> MSGAAAASAAGYDRHITIFSPEGRLYQVEYAFKATNQTNINSLAVRGKDCTVVISQKKVPDKLLDPTTVSYIFCISRTIGMVVNGPIPDARNAALRAKAEAAEFRYKYGYDMPCDVLAKRMANLSQIYTQRAYMRPLGVILTFVSVDEELGPSIYKTDPAGYYVGYKATATGPKQQEITTNLENHFKKSKIDHINEESWEKVVEFAITHMIDALGTEFSKNDLEVGVATKDKFFTLSAENIEERLVAIAEQD;> MTDRYSFSLTTFSPSGKLGQIDYALTAVKQGVTSLGIKATNGVVIATEKKSSSPLAMSETLSKVSLLTPDIGAVYSGMGPDYRVLVDKSRKVAHTSYKRIYGEYPPTKLLVSEVAKIMQEATQSGGVRPFGVSLLIAGHDEFNGFSLYQVDPSGSYFPWKATAIGKGSVAAKTFLEKRWNDELELEDAIHIALLTLKESVEGEFNGDTIE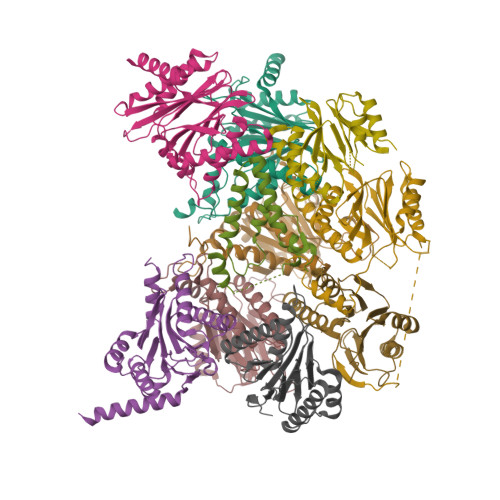LAIIGDENPDLLGYTGIPTDKGPRFRKLTSQEINDRLEAL;> MGSRRYDSRTTIFSPEGRLYQVEYALESISHAGTAIGIMASDGIVLAAERKVTSTLLEQDTSTEKLYKLNDKIAVAVAGLTADAEILINTARIHAQNYLKTYNEDIPVEILVRRLSDIKQGYTQHGGLRPFGVSFIYAGYDDRYGYQLYTSNPSGNYTGWKAISVGANTSAAQTLLQMDYKDDMKVDDAIELALKTLSKTTDSSALTYDRLEFATIRKGANDGEVYQKIFKPQEIKDILVKTGITKKDEDEEADEDMK;> MSGYDRALSIFSPDGHIFQVEYALEAVKRGTCAVGVKGKNCVVLGCERRSTLKLQDTRITPSKVSKIDSHVVLSFSGLNADSRILIEKARVEAQSHRLTLEDPVTVEYLTRYVAGVQQRYTQSGGVRPFGVSTLIAGFDPRDDEPKLYQTEPSGIYSSWSAQTIGRNSKTVREFLEKNYDRKEPPATVEECVKLTVRSLLEVVQTGAKNIEITVVKPDSDIVALSSEEINQYVTQIEQEKQEQQEQDKKKKSNH;> MTSIGTGYDLSNSVFSPDGRNFQVEYAVKAVENGTTSIGIKCNDGVVFAVEKLITSKLLVPQKNVKIQVVDRHIGCVYSGLIPDGRHLVNRGREEAASFKKLYKTPIPIPAFADRLGQYVQAHTLYNSVRPFGVSTIFGGVDKNGAHLYMLEPSGSYWGYKGAATGKGRQSAKAELEKLVDHHPEGLSAREAVKQAAKIIYLAHEDNKEKDFELEISWCSLSETNGLHKFVKGDLLQEAIDFAQKEINGDDDEDEDDSDNVMSSDDENAPVATNANATTDQEGDIHLE;> MNGIQVDINRLKKGEVSLGTSIMAVTFKDGVILGADSRTTTGAYIANRVTDKLTRVHDKIWCCRSGSAADTQAIADIVQYHLELYTSQYGTPSTETAASVFKELCYENKDNLTAGIIVAGYDDKNKGEVYTIPLGGSVHKLPYAIAGSGSTFIYGYCDKNFRENMSKEETVDFIKHSLSQAIKWDGSSGGVIRMVVLTAAGVERLIFYPDEYEQL;> MAGLSFDNYQRNNFLAENSHTQPKATSTGTTIVGVKFNNGVVIAADTRSTQGPIVADKNCAKLHRISPKIWCAGAGTAADTEAVTQLIGSNIELHSLYTSREPRVVSALQMLKQHLFKYQGHIGAYLIVAGVDPTGSHLFSIHAHGSTDVGYYLSLGSGSLAAMAVLESHWKQDLTKEEAIKLASDAIQAGIWNDLGSGSNVDVCVMEIGKDAEYLRNYLTPNVREEKQKSYKFPRGTTAVLKESIVNICDIQEEQVDITA;> MSDPSSINGGIVVAMTGKDCVAIACDLRLGSQSLGVSNKFEKIFHYGHVFLGITGLATDVTTLNEMFRYKTNLYKLKEERAIEPETFTQLVSSSLYERRFGPYFVGPVVAGINSKSGKPFIAGFDLIGCIDEAKDFIVSGTASDQLFGMCESLYEPNLEPEDLFETISQALLNAADRDALSGWGAVVYIIKKDEVVKRYLKMRQD;> MDIILGIRVQDSVILASSKAVTRGISVLKDSDDKTRQLSPHTLMSFAGEAGDTVQFAEYIQANIQLYSIREDYELSPQAVSSFVRQELAKSIRSRRPYQVNVLIGGYDKKKNKPELYQIDYLGTKVELPYGAHGYSGFYTFSLLDHHYRPDMTTEEGLDLLKLCVQELEKRMPMDFKGVIVKIVDKDGIRQVDDFQAQ;> MNIVPQDTFKSQVSTDQDKSVLSSAVPSLPDTLRQQEGGAVPLSTQLNDRHPLESTLKNWETTQRQRQMEQYRQIFGIAEPMKRTMEMEIVNRTDFNPLSTNGSIHRDILLNKECSIDWEDVYPGTGLQASTMVGDDVHSKIEKQLGIGRRIPGLINPWKRRWKKNFIAVSAANRFKKISSSGALDYDIPTTASENLYFQ>SSTCKVPRITTHYTIYPRDQDKRWEGVNMERFAEEADVVIVGAGPAGLSAATRLKQLAAQHEKDLRVCLVEKAAHIG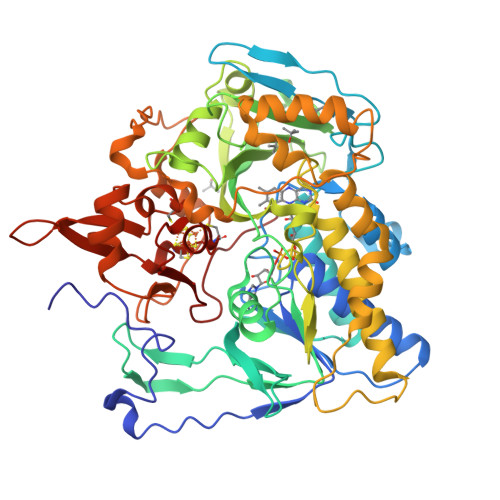AHTLSGACLDPRAFEELFPDWKEKGAPLNTPVTEDRFGILTEKYRIPVPILPGLPMNNHGNYVVRLGHLVSWMGEQAEALGVEVYPGYAAAEILFHEDGSVKGIATNDVGIQKDGAPKTTFERGLELHAKVTIFAEGCHGHLAKQLYKKFDLRANCEPQTYGIGLKELWVIDEKKWKPGRVDHTVGWPLDRHTYGGSFLYHLNEGEPLLALGFVVGLDYQNPYLSPFREFQRWKHHPSIKPTLEGGKRIAYGARALNEGGFQSIPKLTFPGGLLIGCSPGFMNVPKIKGTHTAMKSGTLAAESIFNQLTSENLQSKTIGLHVTEYEDNLKNSWVWKELYSVRNIRPSCHGILGVYGGMIYTGIFYWIFRGMEPWTLKHKGSDSDQLKPAKDCTPIEYPKPDGQISFDLLSSVALSGTNHEHDQPAHLTLKDDSVPVNRNLSIYDGPEQRFCPAGVYEFVPLEQGDGFRLQINAQNCVHCKTCDIKDPSQNINWVVPEGGGGPAYNGM[2x]>MGSDKIHHHHHHMKEALTFDDVLLVPQYSEVLPKDVKIDTRLTRQIRINIPLVSAAMDTVTEAALAKALAREGGIGIIHKNLTPDEQARQVSIVKKTENGIIYDPITVTPDMTVKEAIDLMAEYKIGGLPVVDEEGRLVGLLTNRDVRFEKNLSKKIKDLMTPREKLIVAPPDISLEKAKEILHQHRIEKLPLVSKDNKLVGLITIKDIMSVIEHPNAARDEKGRLLVGAAVGTSPETMERVEKLVKAGVDVIVIDTAHGHSRRVIETLEMIKADYPDLPVVAGNVATPEGTEALIKAGADAVKVGVGPGSICTTRVVAGVGVPQLTAVMECSEVARKYDVPIIADGGIRYSGDIVKALAAGAESVMVGSIFAGTEEAPGETILYQGRKYKAYRGMGSLGAMRSGSADRYGQEGENKFVPEGIEGMVPYKGTVKDVVHQLVGGLRSGMGYIGARTIK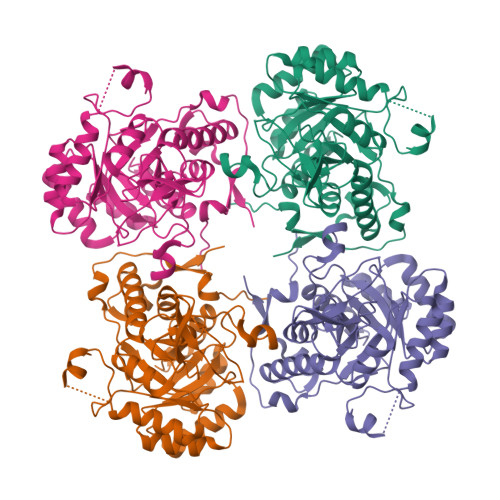ELQEKAVFVKITPAGVKESHPHDIIITKESPNYWVQA[2x]beta-L-galactopyranose | C6 H12 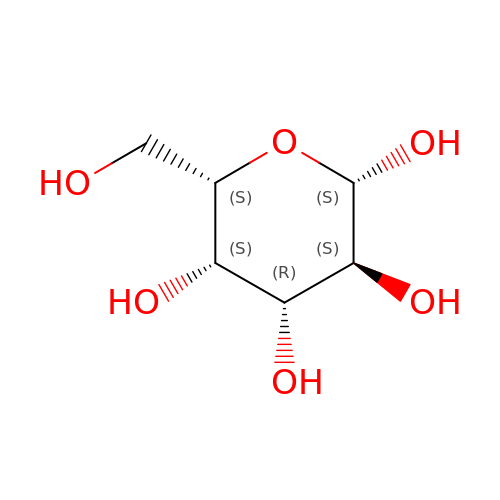O6 | WQZGKKKJIJFFOK-KGJVWPDLSA-N> ANPLYQKHIISINDLSRDDLNLVLATAAKLKANPQPELLKHKVIASCFFEASTRTRLSFETSMHRLGASVVGFSDSANTSLGKKGETLADTIS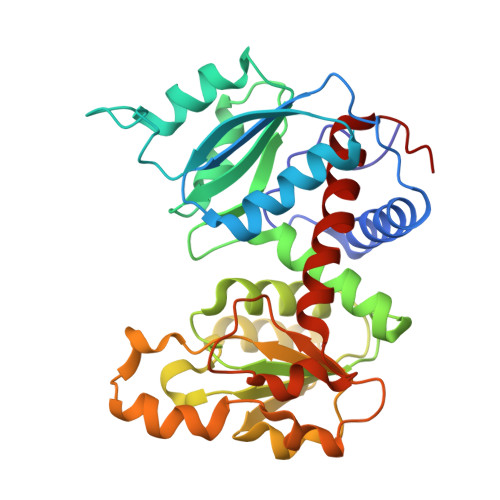VISTYVDAIVMAHPQEGAARLATEFSGNVPVLNAGDGSNQHPTQTLLDLFTIQETQGRLDNLHVAMVGDLKYGRTVHSLTQALAKFDGNRFYFIAPDALAMPQYILDMLDEKGIAWSLHSSIEEVMAEVDILYMTRVQKERLDPSEYANVKAQFVLRASDLHNAKANMKVLHPLPRVDEIATDVDKTPHAWYFQQAGNGIFARQALLALVLNRDLVL> GKRTVRKTKTSKFKWVRNKIDIAEGPGAMNIANVLSTTGGQTIALVGERAFYDPRTAGAAVRCKDLMEIARMPSVFLGESTEPDGRRGYFTWSHTISPVNWVFDDHIYLENMPNLRLFSSCYNYWRGSFVIKLTVYASTFNKGRLRMAFFPNREGAYTQDDAQNAIFVV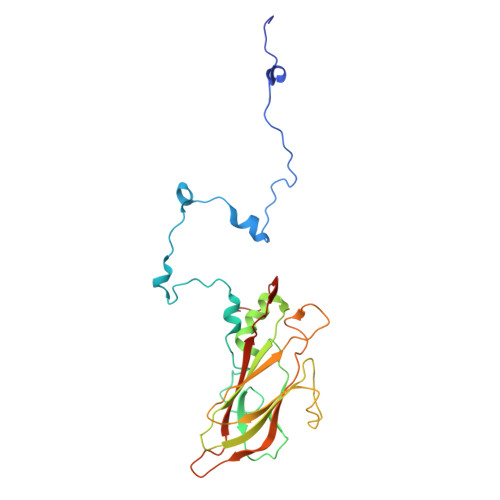CDIGLNNTFEMTIPYTWGNWMRPTRGNSLGHLRIDVLNRLTYNSSSPNAVNCILQIKMGDDAMFMVPTTSNLVMQ> AVANSIVSSVAPGKEPGSLVCIQAKDGKVIGMGARVHCGPATVLVTAGHVLKKGMIADLYLAKYSVSSKEGKRVLMDPTWKIEYGSLNKEADVISVQVPAAVWSRLGVTAARVRKPTVKVPVLAYGGEASGLLQSSQGFATPDGNMSVAHSCSTRPGWAGTPLYAGSDIVAIHRRWEDIGVKNLATNLSIFHANCESSE

Sobemoviruses encode serine-like 3C proteases (Pro) that participate in the processing and maturation of other virus-encoded proteins. Its cis and trans activity is mediated by the naturally unfolded virus-genome-linked protein (VPg). Here, we solved a full Pro–VPg 3D structure of ryegrass mottle virus (RGMoV) that demonstrates the structural changes in three different conformations due to VPg interaction with Pro. The overall fold change of Δ117Pro is typical for CLP and is very similar to the structure of SeMV Pro.

We crystallized and solved 3D crystal structures for two catalytically active forms of Δ117Pro: one in its VPg-free form, the second in its VPg-bound state with fused VPg at the C-terminal part (Δ117Pro-E/A-VPg), and one catalytically defective Δ117Procm form with S159/A mutation. The expression of the Procm variant confirmed the importance of S159 for the catalytic activity of RGMoV Pro. First, in the absence of VPg, L87 shifted towards the VPg-binding pocket. Second, the α1 helix in the VPg-free structure is also slightly shifted towards the empty VPg binding site; although, the position of the catalytic triad H49, located on this helix, is minimally affected. These two conformational shifts are driven by the presence or absence of VPg, since they align well in the Δ117Procm and Δ117Pro cases, which do not contain VPg at all. However, in the Δ117Pro chain B, Δ117Procm, and Δ117Pro-E/A-VPg cases, D92 is directed towards H49, as would be expected in an active Pro. Surprisingly, conformational differences were observed between the Δ117Pro, Δ117Pro-E/A-VPg, and Δ117Procm states, with the only difference being the S159/A mutation. Different crystallization conditions could be at play, but it is very likely that these differences are actual representations of natural conformational oscillations in the Pro molecule.> SMSSFEGQMAEYPTISIDRFDRENLRARAYFLSHCHKDHMKGLRAPTLKRRLECSLKVYLYCSPVTKELLLTSPKYRFWKKRIISIEIETPTQISLVDEASGEKEEIVVTLLPAGHCPGSVMFLFQGNNGTVLYTGDFRLAQGEAARMELLHSGGRVKDIQSVYLDTTFCDPRFYQIPSREECLSGVLELVRSWITRSPYHVVWLNCKAAYGYEYLFTNLSEELGVQVHVNKLDMFRNMPEILHHLTTDRNTQIHACRH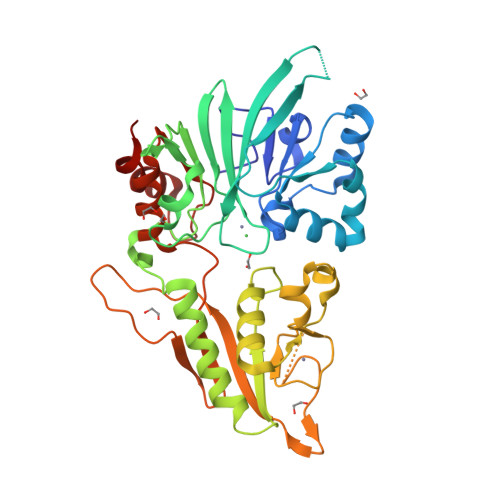PKAEEYFQWSKLPCGITSRNRIPLHIISIKPSTMWFGERSRKTNVIVRTGESSYRACFSFHSSYSEIKDFLSYLCPVNAYPNVIPVGTTMDKVVEILKPLCRS> YFGKLESKLSVIRNLNDQVLFIDQGNRPLFEDMTDSDCRDN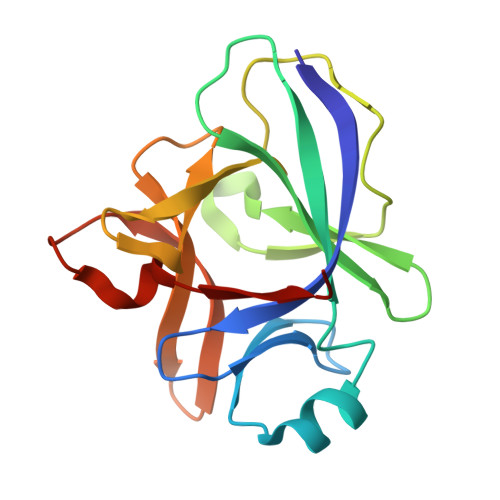APRTIFIISMYKDSQPRGMAVTISVKCEKISTLSCENKIISFKEMNPPDNIKDTKSDIIFFQRSVPGHDNKMQFESSSYEGYFLACEKERDLFKLILKKEDELGDRSIMFTVQNED> GENLYFQHMRHFARTHAIGQIVPGKVTKLVPFGAFVRVEEGIEGLVHISELAERHVEVPDQVVAVGD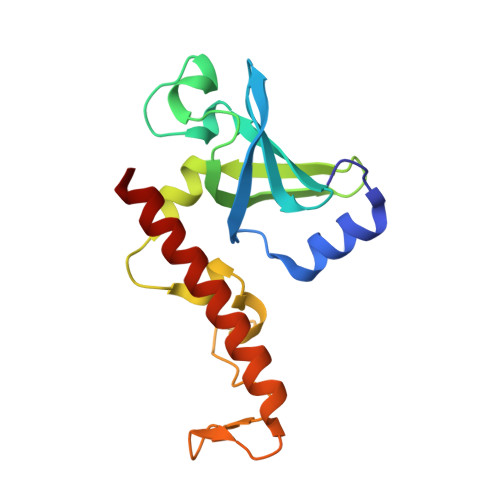DAMVKVIDIDLERRRISLSLKQANEDYTEEFDPAKYGMADSYDEQGNYIFPEGFDAETNEWLEGFEKQRAEWEARYAEAERRHKMHTAQMEK> ISGGDAIYSSTGRCSLGFNVRSGSTYYFLTAGHCTDGATTWWANSARTTVLGTTSGSSFPNNDYGIVRYTNTTIPKDGTVGGQDITSAANATVGMAVTRRGSTTGTHSGSVTALNATVNYGGGDVVYGMIRTNVCAEPGDSGGPLYSGTRAIGLTSGGSGNCSSGGTTFFQPVTEALSAYGVSVY;> VDCSEYPKPACTFEYRPLCGSDNKTYGNKCNFCNAVVES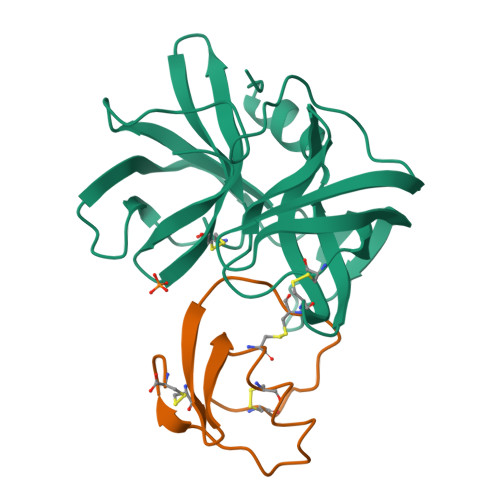NGTLTLSHFGKC> EAERVRVFHKQAFEYISIALRIDEDEKAGQK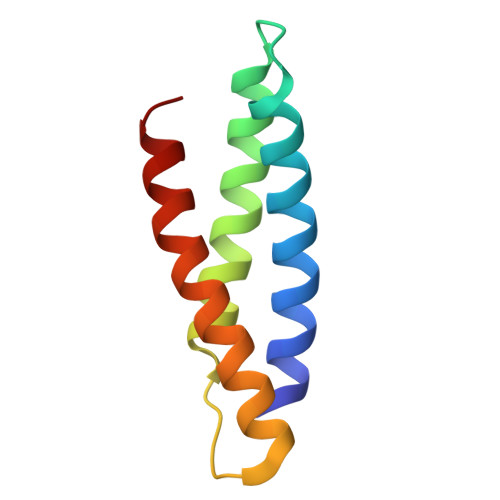EQAVEWYKKGIEELEKGIAVIVTGQGEQCERARRLQAKMMTNLVMAKDRLQLL>GSSHH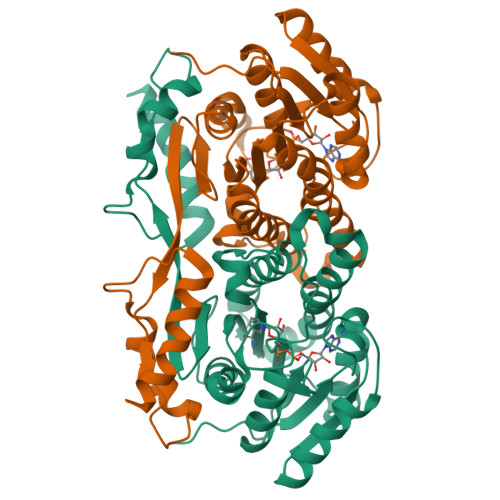HHHHSSGRENLYFQGHMGSPLRFDGRVVLVTGAGAGLGRAYALAFAERGALVVVNDLGGDFKGVGKGSLAADKVVEEIRRRGGKAVANYDSVEEGEKVVKTALDAFGRIDVVVNNAGILRDRSFARISDEDWDIIHRVHLRGSFQVTRAAWEHMKKQKYGRIIMTSSASGIYGNFGQANYSAAKLGLLGLANSLAIEGRKSNIHCNTIAPNAGSRMTQTVMPEDLVEALKPEYVAPLVLWLCHESCEENGGLFEVGAGWIGKLRWERTLGAIVRQKNHPMTPEAVKANWKKICDFENASKPQSIQESTGSIIEVLSKIDSGS[6x]>MDQKLLTDFRSELLDSRFGAKAISTIAESKRFPLHEMRDDVAFQIINDELYLDGNARQNLATFCQTWDDENVHKLMDLSINKNWIDKEEYPQSAAIDLRCVNMVADLWHAPAPKNGQAVGTNTIGSSEACMLGGMAMKWRWRKRMEAAGKPTDKPNLVCGPVQICWHKFARYWDVELREIPMRPGQLFMDPKRMIEACDENTIGVVPTFGVTYTGNYEFPQPLHDALDKFQADTGIDIDMHIDAASGGFLAPFVAPDIVWDFRLPRVKSISASGHKFGLAPLGCGWVIWRDEEALPQELVFNVDYLGGQIGTFAINFSRPAGQVIAQYYEFLRLGREGYTKVQNASYQVAAYLADEIAKL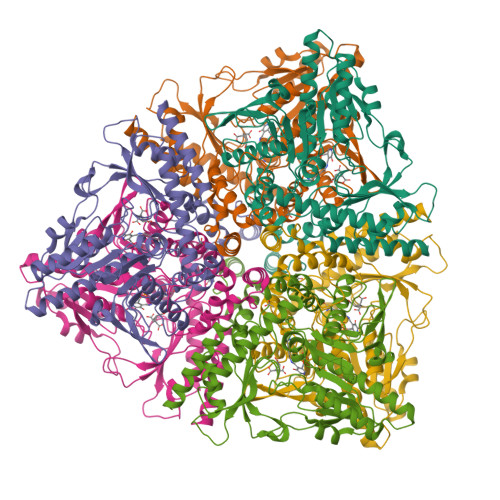GPYEFICTGRPDEGIPAVCFKLKDGEDPGYTLYDLSERLRLRGWQVPAFTLGGEATDIVVMRIMCRRGFEMDFAELLLEDYKASLKYLSDHPKLQGIAQQNSFKHT[2x]> MQSNKTFNLEKQNHTPRKHHQHHHQQHHQQQQQQQQQPPPPIPANGQQASSQNEGLTIDLKNFRKPGEKTFTQRSRLFVGNLPPDITEEEMRKLFEKYGKAGEVFIHKDK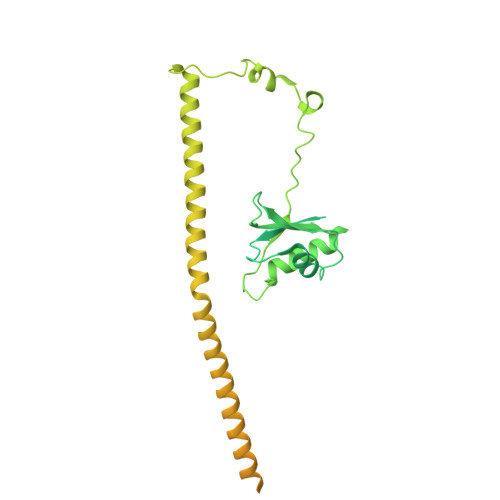GFGFIRLETRTLAEIAKVELDNMPLRGKQLRVRFACHSASLTVRNLPQYVSNELLEEAFSVFGQVERAVVIVDDRGRPSGKGIVEFSGKPAARKALDRCSEGSFLLTTFPRPVTVEPMDQLDDEEGLPEKLVIKNQQFHKEREQPPRFAQPGSFEYEYAMRWKALIEMEKQQQDQVDRNIKEAREKLEMEMEAARHEHQVMLMRQDLMRRQEELRRMEELHNQEVQKRKQLELRQEEERRRREEEMRRQQEEMMRRQQEGFKGTFPDAREQEIRMGQMAMGGAMGINNRGAMPPAPVPTGTPAPPGPATMMPDGTLGLTPPTTERFGQAATMEGIGAIGGTPPAFNRPAPGADFAPNKRRRY>[2x]MSLRPCFVSLIDESDKPILIYVPNEAENEMNDVLKYNVLSNISLDYFESALVEWHSLDSKPLLKSIFQLEGVSVFAMLIKQTGLKIVIGFEQKSLSGADDEFEAINQIFETVRKIYIRVKCNPLLVSGDEKSIIKSLERKFDELFISTEVEL;>MSSTHSNNVGHPQSSPQGPLTEQQRAQQQYQIFENSLPKVSQSVYQMLLNEMVPLAMGIERQISGDVISSDSNVTSENGNINNMIKRLKIEEHHTVDIIRSHNLIHELYKADEEEKEKVLARLRNIGFQIGLKLSELLIFSNNPNLKFKEMDLLLIMKFICRDVWKQIFGKQIDNLKTNHRGTFYLLDYDYRPIQSFSLEEDAKNEELKMIEPFLEIPVGIIRGVLSSLGYSSEEVICLASFIDRPTDRPKTAFPKGVSFHVQVTMPQ[2x];>MVSTTQSRSLKAMGEEIWKNKTEKINTELFTLTYGSIVAQLCQDYERDFNKVNDHLYSMGYNIGCRLIEDFLARTALPRCENLVKTSEVLSKCAFKIFLNITPNITNWSHNKDTFSLILDENPLADFVELPMDAMKSLWYSNILCGVLKGSLEMVQLDCDVWFVSDILRGDSQTEIKVKLNRILKDEIPIGED[4x];>MGIYSFWIFDRHCNCIFDREWTLASNSASKQNEEDAKLLYGMIFSLRSITQKLSKGSVKNDIRSISTGKYRVHTYCTASGLWFVLLSDFKQQSYTQVLQYIYSHIYVKYVSNNLLSPYDFAENENEMRGQGTRKITNRNFISVLESFLAPMVNQ[2x];>MAIETILVINKSGGLIYQRNFTNDEQKLNSNEYLILASTLHGVFAIASQLTPKALQLTQQTNIENTIPYIPYVGMSSNRSDTRNGGGNNNKHTNNEKLGSFKGDDFFKEPFTNWNKSGLRQLCTDQFTMFIYQTLTGLKFVAISSSVMPQRQPTIATTDKPDRPKSTSNLAIQIADNFLRKVYCLYSDYVMKDPSYSMEMPIRSNLFDEKVKKMVENLQ[2x];>[2x]MSQRIIQPSASDQQFPGKSDGYEYTVGPKQAITSEASTTYIPSRIYSESLLFKRQEASLSAMAFLFQEMISQLHRTCKTAGDFETKLSDYGHNIGIRLLELLNFRASSSPSSLPRASAFLSQNESSSKLSNASNSPGMLANSSTATSASANERLQEKQTESLSNYITKMRRRDLKILDILQFIHGTLWSYLFNHVSDDLVKSSERDNEYMIVDNFPTLTQFIPGENVSCEYFVCGIIKGFLFNAGFPCGVTAHRMPQGGHSQRTVYLIQFDRQVLDREGLRFG;>[2x]MPQYFAIIGKKDNPVYEIEFTNAENPQGFPQDLKELNPFILHASLDIVEDLQWQINPTSQLNGNGGNGSNGGGGFLRSRAVNNTDNCYLGKVDHFYGLAITAYISYSGMKFVMIHGNSANSSVVIDDNNMRSFYQEVHELYVKTLMNPFYKITDPIRSPAFDSRVRTLARKHLSK;>MDKEIYCGSVPVSYFDPFDLFESLRPEFQQILPLDNIHWKAFDGTVRTVNRLPIELIPEGRGEADKSNDEQPFIRFLIVNCISIDQYRAKVRPLVRQWLPNLESVSSSTGEKMIYKPIILLYANSEVVDSNLFKSVSLMEKFGKDFPHVQTLEVRSVYRSPKERQEFWNQFSQKIKASVLSIFQKRLTHLQHSLANLQKGNNFEEQLLTREKLYELYVVFNILEDASLELQKIKKEILRRNMNMPDGKLQVPFESSSKSDESLGSIIIEGTLDKFQLHKYFFIRRLRLLKLEDQTLTAFVGAFQLIKNFIESISIEYRKSVRLLEFKHYFITSMLSYFEFENVSNPLLCEIKAELLMLKRDNWVQGVMATSGYRLMDKNYPNSDVKYKFDLLKETFVDETVFQENFLTLTKEILSLFNKCEGKRQRIVDILSIEIGLLYYQGKKYEEAVSLFLSCYEYYTQTNKNSIGLKILQVFIDSLSHCPKLDVLQIDGESVSASAVLTNAFLNILKLCKDNDSKEIWWKKFMDLQMKNNIHLMYPLDGLFEVTLNSKVHLARANVSAIEVNLKSYGFPEDISTKTMRLSLKNMGGDVIVFGASDFLLKKGENKLILECRDIMYGEFSLLSFEIIVEGITFVKEFPENQDEFIVVPEIYCKESTKVLVKQAHNLNLGEYALELKSVQSDALESLQVEVEVQKNIGNMKNLPVSFSMDEIQARKRYNTPFENVRLEYYLLDQITAFDLIIKTSFTKKNDQGTFGETKKVRIQCYLQLSVSVEDIFKKDIFFFKFLLNSSVREEPVILYSSELSAPDTRNDYNIRGDYIATTPALITFDGNESFINCYEITANNNFDSKDIFNLKVRYNTLKEQLDCFITDAVLIEGDVEWFI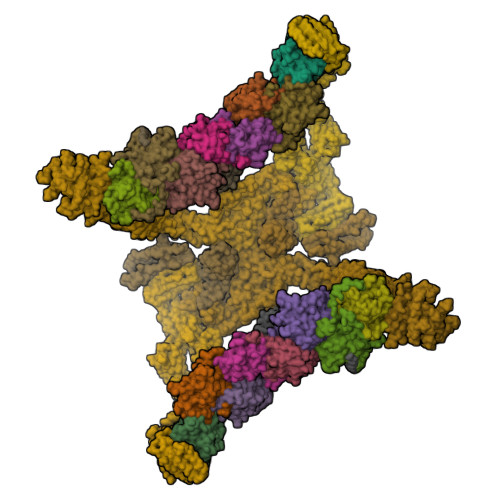LFEKWKTFWELEILKKLKYDYDAFKENRIIRLLKTSIDLNKTKSKIRNLCIEKAVLDKILICLNKVSRGIAVCNTDMDEYVRNLVPKQLTVPVQLPGFEQFFHVQFEQMETSHDALHDTIATIGNSLSYTVIVENLSGQWGQDVIDDGGYIFEILSSNEWLIHGQKRCAIKEKRKEFEVHLIPLKKGYLNFPRVEITNINGKSCRVDHSNAFESILIF[2x];>[2x]MNILKHFPSYVGPSKIRTLVIPIGHWTRKEFNNAVQKLSEFNEIHLSDVTPIDSPIFTPQGFPHGKLFFDFLTIDHDDALELFLYDFEPFRKTFVIIGLVNDYSDPLTNLNFMKEKYPTLISPNLVYASSTPTKELEQTIDTMENVFASSPDMQKNIETIMCDIARNFLTALNSYYSSYKHVTLRSPGAIGGNAVLKTTLIRQNSYTSSSSSTPMSAVQSSVSSSSKAGSVTTASKRLSSFEMTTNSLKRSASLKLATTLSTSENRSQQKSLGRQMKILGNFQLLAGRYVDALNSFVDAITTLYKVRDYLWLGSALDGISICFLLLSYLGLSYQIPQIVSLICPVEKLNFESSSTGISPVDSNSKATASTTASSTPRNSISIAAMQSPRNSIMSLSAPALNIDVENINLPLLIKCISDKVLYYYDLSLMHNSEYAPQVVYCEFLLKTLTFMTSCYKSSEFSKDVLDNIVKNQHRALSDIPNSPMFPRFEVYFYSNKLFELQLKEMQVEAQIKIYSTMAEVYRLLGYKRKQLFVLRLLMVALLATPNKIAWHPDYRTLIDTIIELLNINESEAKINVDDPSQSTWLILQKKILQLCIKVSRKINDFEYVAKFSSILITKYTHLLNQSEQDALFKEYIQPSITNESITSYWDPFILREVVINRILDSDPTSNEIPLESDVSSLESLENRQKTQDINPQEVFNPFKRVQPTSFVSNNSTKVPILVFLVGDKAEFTCRVQNPFKFDFTINDIQLDEEISEFCEIDRKAVSYSGPYNVKAESIRSITLPLIIKKPTYKKIYEISCLKISILKLPLQKFDIINDSRRSNPVEEEAEYSKCIYGKLKIKILPEQPQLELLSTSKMTRNSWMMLDGTKTDFHITVRNKSLSCAINHIKIIPMNNIEQMLKPDYWKKMPPDDLYIMEKQLDWLSKSCVRIIKLPTVIKPNETITFDLELDNTAVPFNFTGFDLLIEYGMSATDESCIYLKKLSIPYEVTLRRTIEVPSMDIIPLNELFSSQVENVDWIEYVMSKIRAESNLHSRDFILLLLDFRNSWIDGIKLNVQFEDFTSNEYHVEASHTSRIIVPIKKIDYKKYNFENTPIPRIFPGRQFIQSGLNEEQTIEMRQKFWCREHIISKLKCNWKLTTDQSVTGSVDFNKFIEKFDHKMVYTIYPGRLFYGVQLLLDEPKVKVGEIINLKIITEPTSTCRRKQNSTVNFLDIVIFDSKTSKILPRSNRRILYNGSLTKPISTTKVSEINLEIIPIEKGRYEFSVCISKSNNQDGIIQFDSENVILSVI;>MECFVPLRCDLDGSNIEQLRQSHLSRKFIIFDEQLNLWLWFQGNSQENKRFVLQNMIILINEAQVTRTSTIDDYFTQVENNENLWRLKNDCCSKILFKSNVVMNNGYNNQIKFVFEYKSVDANFNNQDSLQDPQAKYTLDKYSSEEILPSFEPVYSWSSAATKSSKNTNNHLEKNNRATHRVSSKNSEVHEADVSRNPNTFTLKLQYPIFSLLNMRLRNISLKSEHCILSSLDFQTSKASEQLTKKFIYPQEHNSFLKLNFQEISYKLIDGTSQIELDPICPLKVPLTAFSYDSISATFKLVLLPKSTQPHRVKITLAYELELHPNLKLPVRTSWETEVTLKRSMPISSTSSQYSSNNNNTNHSASFNGAANNVNSGGLANLRLGGVSSSRFSLGAASTTSLVNSKLSNVKFKFINSNIKVIKGEKFTMRLQIINSSSSPLDLVVYYNNTINPIPSANNVRNSNGINNCGMNNGTIPNSPLTLENQYQLHNKYRKIAEGIILLSNDYKIPVVPPRETYFADLRFIGIMSGYYGTLSGLKVLDLNTNELIEVGNGASVLIQ[2x];>[2x]MSNEDYGYDYDYLFKIVLIGDSGVGKSNLLSRFTTDEFNIESKSTIGVEFATRTIEVENKKIKAQIWDTAGQERYRAITSAYYRGAVGALIVYDISKSSSYENCNHWLTELRENADDNVAVGLIGNKSDLAHLRAVPTDEAKNFAMENQMLFTETSALNSDNVDKAFRELIVAIFQMVSKHQVDLSGSGTNNMGSNGAPKGPTISLTPAPKEDKKKKSSNCC>ETTPTTVNGGTVHFKGEVVNAACAVDAGSVDQTVQLGQVRTASLKQTGATSSAVGFNIQ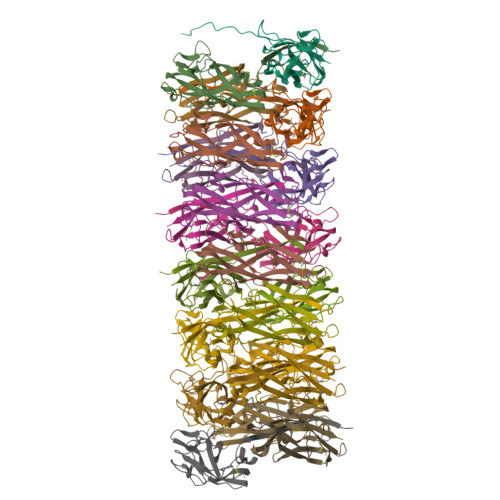LNDCDTSVATKAAVAFLGTAIDSAHPKVLALQSSAAGSATNVGVQILDRTGAELTLDGATFSVQTTLNNGTNTIPFRARYYAIGEATPGAANADATFKVQYQ[21x]> MSKQLTFISAGATAAVLQSASAIVSKVAGGRVQTKTAKEAGRHAVVVGPETPIGVHTAVTEVPKSAQDPLFSGVSTVVVRAVLPRAAPDSVQLRDALDVYASAGIDTKEEVRSATEAFKKSAEVAVGKAKAKGVKRIVLVVK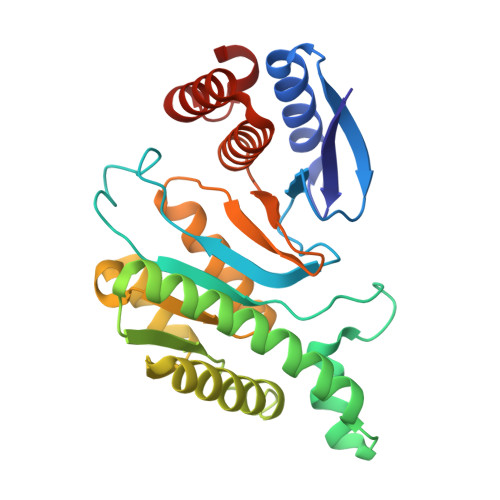QASKHNCINELFKKISTETIESAGLTTEVVGTAAVANQLIVNPESLGVVLLNDVAATEQIELAFAGVVGGVSRVYHTVEGGKISAGHSFKSVALAVAQELRELGLSSEADKVEAAASKNPRAVVSAL>[10x]MEGLNLVATALAVGLGAIGPGVGIGIIVSGAVQAIGRNPEIENRVVTYMFIGIAFTEALAIFGLVIAFLIGFGVLQ;>MSTRTRNILIIVGALIISIASRFFLYTGPPHVEVAAEVIFDGIPGFPITNSFVVAIIIDIFVIALAVAATRNLQMVPRGLQNVMEFILESLYNLFRNINAKYVATAFPLVATIFLFVLFGNWFGLLPGVGSIGVCHEKKEEHAVVDERLALAAPAAPLSSVAAAEGEEIHDTCAAQGKKLVPLFRAPAADLNFTFAIAVISFVFIEYWGFRALGPGYLKKFFNTNGIMSFVGIIEFISELVKPFALAFRLFGNIFAGEVLLVVMAFLVPLLLPLPFYGFEVFVGFIQALIFALLTYAFLNIAVTGHDEEHAH[2x];>[4x]MEALGINPTLFIAQLINFLLLIFILRALLYRPVMNLLNERTRRIEESVRDAEKVREQLANARRDYEAEIARARQEAAKIVAQAQERAKQQEA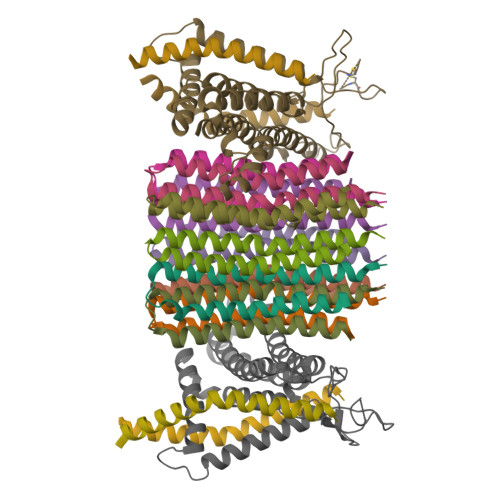EIIAQARREAERLKEEARAQAEQERIRMLSEAKSQIADLVTLTASRVLGAELQARGHDALIAESLAALDRRN>KLFITEGYEVGRVNGLAVIGESAGIVLPIIAEVTPSMSKSEGRVIATGRLQEIAREAVMNVSAIIKKYTGRDISNMDVHIQFVGTYEGVEGDSASISIATAVISAIEGIPVDQSVAMTGSLSVKGEVLPVGGVTQKIEAAIQA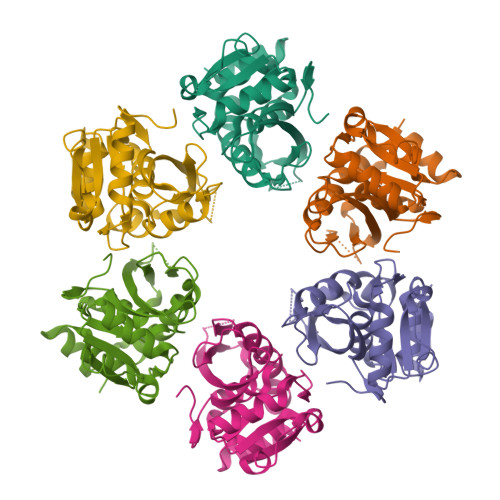GLKKVIIPKDNIDDVLLDAEHEGKIEVIPVSRINEVLEHVLEDGKKKNRLMSKFKELELAAV[6x]> 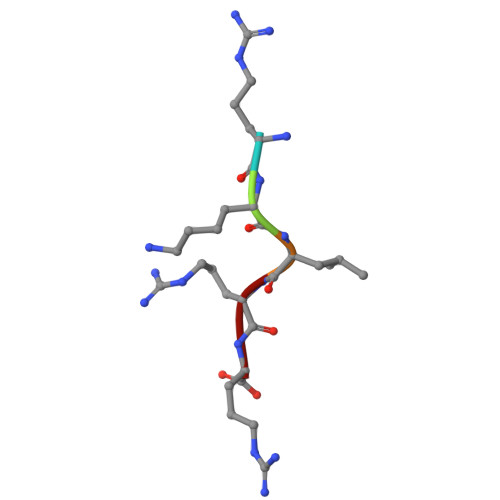RKLRR>MGKSELSGRLNWQALAGLKASGAEQNLYNVFNAVFEGTKYVLYEKPKHLKNLYAQVVLPDDVIKEIFNPLIDLSTTQWGVSPAFAIENTETHKILFGEIKRQDGWVEGKDPSAGRGNAHERSCKLFTPGLLKAYRTIGGINDEEILPFWVVFEGDITRDPKRVREITFWYDHYQDNYFMWRPNESGEKLVQHFNEKLKKYLD[2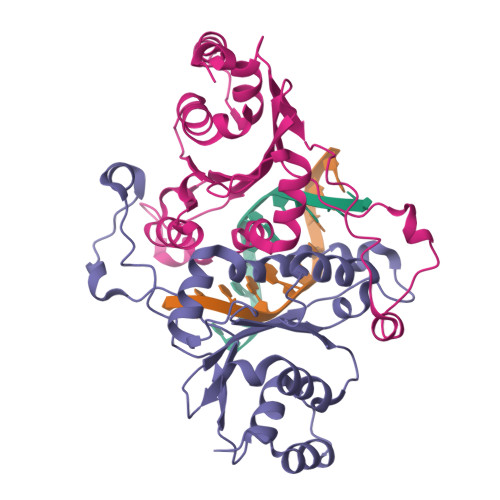x]The high affinity interaction between γH2AX and the tandem BRCT domain pair (BRCT2) module at the C-terminus of MDC1 (0.4 μM, in vitro) is a key step in the amplification and spreading of the γH2AX signal via recruitment of MRN and ATM, which in metazoan cells also facilitates recruitment of 53BP1 and the associated Shieldin complex to DNA double strand breaks, through ubiquitylation of histone H2A. Although no MDC1 homologue is evident in S.cerevisiae, Mdb1 in S.pombe has a similar molecular architecture and shares the ability of MDC1 to interact with the equivalent γH2A modification via its C-terminal BRCT2 module. However, unlike MDC1, which is essential for genomic stability, Mdb1 appears to be largely dispensible. Surprisingly, despite strong conservation on both sides, no interaction was observed between the single SDT motif present in Mdb1, the S.pombe homologue of MDC1, and any part of Rad4, the S.pombe homologue of TOPBP1.

Since its discovery, phosphorylation of the most C-terminal serine residue (Ser 139) in the histone H2A variant H2AX has become the definitive biomarker for the presence of DNA double-strand breaks (DSBs) in mammalian cells. Comparable phosphorylations of closely related C-terminal motifs are also observed in both of the yeast species commonly used in genome stability studies, Saccharomyces cerevisiae and Schizosaccharomyces pombe but here the phosphorylation occurs on the normal histone H2A isoform rather than a specialised variant. However, subsequent studies demonstrated that γH2AX is a direct participant in recruitment of repair factors, and interacts directly with MDC1; via specific binding of its C-terminal tetrapeptide incorporating pSer139, to the tandem BRCT domain at the C-terminus of MDC1. This, and the earlier demonstrations of phosphorylation-dependent interactions of BRCA1 and PTIP, highlighted the key role played by BRCT domains in mediating interactions between proteins involved in the DNA damage response. Structural analysis of the Crb2-BRCT2 module revealed a similar mode of interaction with the C-terminal phosphopeptide motif of γH2A as that seen in the interaction of MDC1-BRCT2 with MDC1, allowing the identification of key features in the BRCT2 module that mediate the specificity for the phosphorylated serine and carboxyl-terminus. Critical to the ability of BRCT domains to recognise the phosphorylated status of ligand peptides, are a triplet of amino acids (Ser548, Arg558 and Lys619 in Crb2) which make multiple hydrogen binding and charge-neutralising interactions with the negatively-charged phosphate group of the phosphorylated peptide.

>[2x]MNKHTNLVTSSFNLTKPMKSFIRRNGLRVQESVTDETDFVILGSPPLRRTHKFLLATSLGIPLVSSQYLTDCIKSGKVLDFRSYKYKDEEAEAKWGFRLDDIHRRTCFNGKRLYITKAIRDSMVGDSIHGLYSILETSGAEIVGDIKRAQEKDTIILAQPDNDQEGRNMSATGLNVYKIELVALSILRDRIDFDEFLID;>SGRTGKPSQEL[2x]> LPQSVSRAAITAAYRRPETEAVSMLLEQARLPQPVAEQAHKLAYQLADKLRNQKNASGRAGMVQGLLQEFSLSSQEGVALMC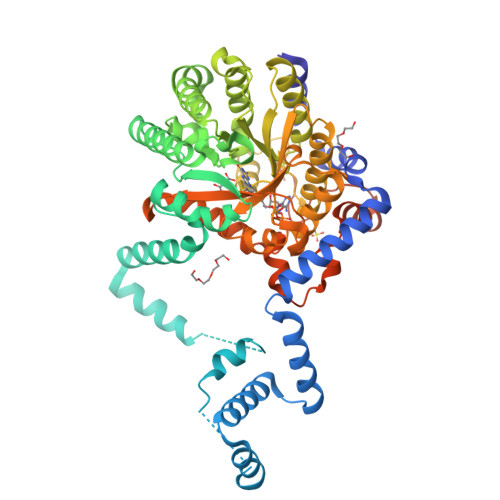LAEALLRIPDKATRDALIRDKISNGNWQSHIGRSPSLFVNAATWGLLFTGKLVSTHNEASLSRSLNRIIGKSGEPLIRKGVDMAMRLMGEQFVTGETIAEALANARKLEEKGFRYSYDMLGEAALTAADAQAYMVSYQQAIHAIGKASNGRGIYEGPGISIKLSALHPRYSRAQYDRVMEELYPRLKSLTLLARQYDIGINIDAEESDRLEISLDLLEKLCFEPELAGWNGIGFVIQAYQKRCPLVIDYLIDLATRSRRRLMIRLVKGAYWDSEIKRAQMDGLEGYPVYTRKVYTDVSYLACAKKLLAVPNLIYPQFATHNAHTLAAIYQLAGQNYYPGQYEFQCLHGMGEPLYEQVTGKVADGKLNRPCRIYAPVGTHETLLAYLVRRLLENGANTSFVNRIADTSLPLDELVADPVTAVEKLAQQEGQTGLPHPKIPLPRDLYGHGRDNSAGLDLANEHRLHHHHHH> MKRYRSSVVTRLVRAITLRPDATVDPERYPLGYVPLDGSESVDSVWSLVKSGAFVAPLSKIETIHRAHVGIRYLTQSEYPALSSIDVVGLQTRLKELCSRLLIRRDFWVLDDYNDPELNSSF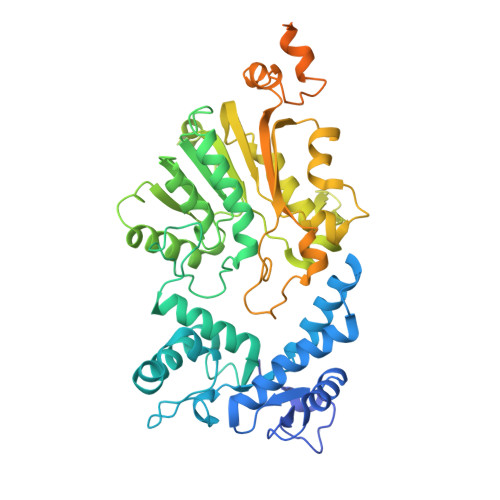GIQNMYFDNFKWSQVLWRRFQQYVEEYFPVAEHTHLTYDEYLQLLRSFSHFEQGAKLLPLLPKRYRIHPPFGVPALSRIDMEPLLLYSQWLKNFRGPLKLDAALVIRSGCGAAVFATKLNGVPIVRGVDPNPRAVMSCRKDAQRMGRRFDSISFRVGEMFPDKDDGNGVPNSRKYDIIVFYPDQGCYNLFFTNAIGEYAPVLTGFAGTLEHFFEEAGDYLSDSGVIVLCCTNVYSILKPTEPHPIEYEIKVNRRWVLLDYYDMPVRGKGTLSHTPTDHHYRIPMEMRKCMRSELWVLHKMTSIAHFAHIHNIPGAQPPSCVVSHWRNKAIGKLRRAVLKGQVESSGGDWDDYKKRLVHLLQEQSENDEDDKAQAIRMAMDPNYPKELADRARAAIEKNMDTDKAFHNNVAKAFGDISPRERFDAYLSCYRL Gram-negative bacteria from the Bacteroidota phylum possess a type-IX secretion system (T9SS) for protein secretion, which requires cargoes to have a C-terminal domain (CTD). The T9SS is a specialized OM shuttle of protein cargoes that includes a rotary motor, a translocon, an OM-associated scaffold and an attachment complex. T9SS transport requires a C-terminal domain (CTD) of 70–100 residues, also known as the ‘T9SS signal’, which contrasts with the short unstructured signal peptides of other secretion systems. The CTD is apparently necessary and sufficient for T9SS secretion.

Eventually, the structure was solved in the primitive space group P3121 by single-wavelength anomalous diffraction (SAD) with data collected at the selenium K-edge, but it could only be refined in P31 after the diffraction data had been detwinned. All this notwithstanding, the final structure, with six protomers in the crystallographic asymmetric unit (a.u.), was backed by solid Fourier map density and exhibited good validation parameters. The two LKK sheets are arranged with an intersheet angle of ~35° and have Greek-key connectivity. Finally, the C-terminal segment of strand β7 encompasses the sequence K787–L–I–K–K791, which is found at the C-terminus of five unique serine- and metal-dependent peptidases secreted by the T9SS of T. forsythia in addition to mirolase, collectively named ‘KLIKK-peptidases’. Structure similarity searches with LKK identified the CTDs of PorZ (Z-score 10.0, rmsd 1.7 Å, 72 aligned residues, 18% identity; see [75]) and PorU (Z-score 9.9, rmsd 1.9 Å, 78 aligned residues, 19% identity) as the closest structural relatives. We found that, in addition to the much longer Lβ2β3, LKK lacked one residue in motif Lβ3β4, which is relevant for T9SS function in P. gingivalis (see §2.3), and the conserved glycine was replaced with methionine. Moreover, the mutant strain evinced substantially less extracellular PPAD activity. This confirms that the CTDs are not functionally interchangeable between P. gingivalis and T. forsythia due to the disruption of motif Lβ3β4, despite both species belonging to the Bacteroidia class.

>[6x]GSLTLSPNPATDVVTLQLTETDEVSGLSVLSTERSAYEIQIWSGMRMLRSFRTNEPTFQIPMAGLPAGLYFVRVVKNGQTYTQKLIKK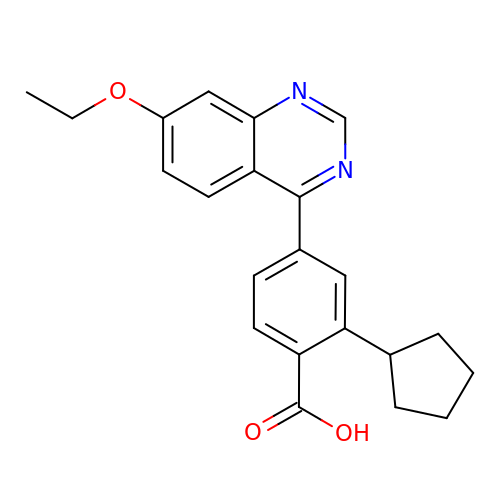(4M)-2-cyclopentyl-4-(7-ethoxyquinazolin-4-yl)benzoic acid | C22 H22 N2 O3 | LIZGTJPPOJGDHW-UHFFFAOYSA-N>[6x]MTSAEMTSPNNNSEHQAIAKMRTMIEGFDDI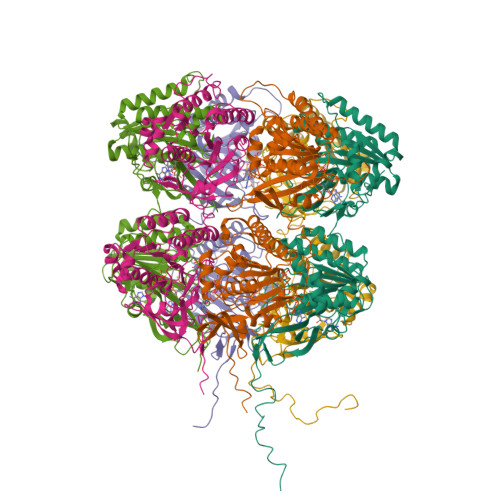SHGGLPIGRSTLVSGTSGTGKTLFSIQFLYNGIIEFDEPGVFVTFEETPQDIIKNARSFGWDLAKLVDEGKLFILDASPDPEGQEVVGGFDLSALIERINYAIQKYRARRVSIDSVTSVFQQYDASSVVRRELFRLVARLKQIGATTVMTTERIEEYGPIARYGVEEFVSDNVVILRNVLEGERRRRTLEILKLRGTSHMKGEYPFTITDHGINIFPLGAMRLTQRSSNVRVSSGVVRLDEMCGGGFFKDSIILATGATGTGKTLLVSRFVENACANKERAILFAYEESRAQLLRNAYSWGMDFEEMERQNLLKIVCAYPESAGLEDHLQIIKSEINDFKPARIAIDSLSALARGVSNNAFRQFVIGVTGYAKQEEITGLFTNTSDQFMGAHSITDSHIDTITDTIILLQYVEIRGEMSRAINVFKMRGSWHDKAIREFMISDKGPDIKDSFRNFERIISGSPTRITVDEKSELSRIVRGVQEKGPES>[2x]FLKSXALL

Novo29 is an eight-residue depsipeptide comprising a macrolactone ring and a linear tail. Novo29 kills bacteria by inhibiting bacterial cell-wall synthesis, with no detectable resistance occurring upon serial passaging. We also report the X-ray crystallographic structure of a hydroxyAsn epimer of Novo29 (epi-Novo29), which may provide insights into how Novo29 binds bacterial cell-wall precursors.

The crystallographic phases were determined using single-wavelength anomalous diffraction (SAD) phasing from the incorporated iodide ions. Novo29 did not form crystals from any of the conditions tested. epi-Novo29 formed rod-shaped crystals from 2.8 M sodium acetate at pH 7.0. Further optimization in a 24-well plate format afforded long rectangular crystals suitable for X-ray diffraction from 2.8 M sodium acetate at pH 6.6. The asymmetric unit contains two molecules of epi-Novo29, which exhibit only minor differences in conformation. In the X-ray crystallographic structure, epi-Novo29 adopts an amphiphilic conformation, with the side chains of Phe1, d-Leu2, Leu7, and Leu8 creating a hydrophobic surface and the side chains of d-Lys3, Ser4, and (2R,3S)-hydroxyAsn5, as well as the N-terminal ammonium group, creating a hydrophilic surface. An intramolecular hydrogen bond between the main-chain NH group of Ala6 and the side chain OH group of Ser4 helps enforce this conformation. In the lattice, epi-Novo29 packs so that the hydrophobic surfaces come together, with four sets of epi-Novo29 molecules forming a hydrophobic core. The macrolactone ring of epi-Novo29 adopts a conformation in which the main-chain NH groups of (2R,3S)-hydroxyAsn5, Ala6, Leu7, and Leu8 converge to create a cavity, which binds ordered water and acetate anion. In contrast, epi-Novo29 exhibited no MIC activity (>32 μg/mL) against any of the bacteria, thus indicating that the 2R,3R stereochemistry of the hydroxyAsn residue is critical to the antibiotic activity of Novo29.> DRRHVLLQAEFYQRSEGPDKAWAQFGFHFDADELFHVELDAAQTVWRLPEFGRFASFEAQGALQNMAVGKQNLEVMISNSNRSQQDFVTPELALFPAEAVSLEEPNVLICYADKFWPPVATMEWRRNGAVVSEGVYDSVY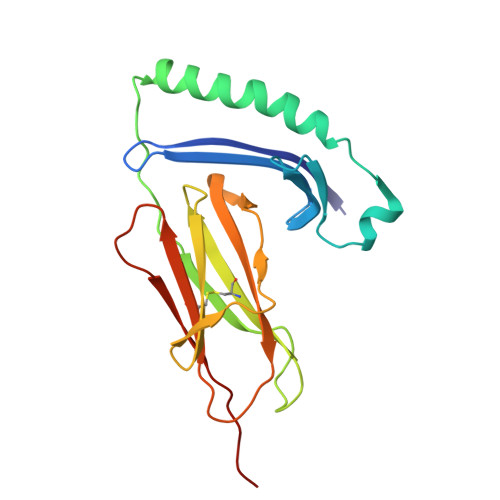YGRPDLLFRKFSYLPFVPQRGDVYSCAVRHWGAEGPVQRMWEPEVPEPPSE>MGPIPPTGVPVGDFFVCGRMTTLHMGGQSGIQATTLVNGMIYRTDHPEPSTSPVSNWEFTVLENNTIVGAGMGCVWFQKSEALVWTLDGQKLSGWNTLDGVGTTQLTVAWRQHNRTIYGWANVVAWNSEEWHTNAEQPHQPILRLTYWLVKINVLSEPEDFDVVQKSPLAYLEDYTTAQSKSAIQKLNFQTFQKPEGGGTLRAQYSTTPRQGDFAVIWQIGRHNFDMSTGKGTPVESLSDYVMPQQ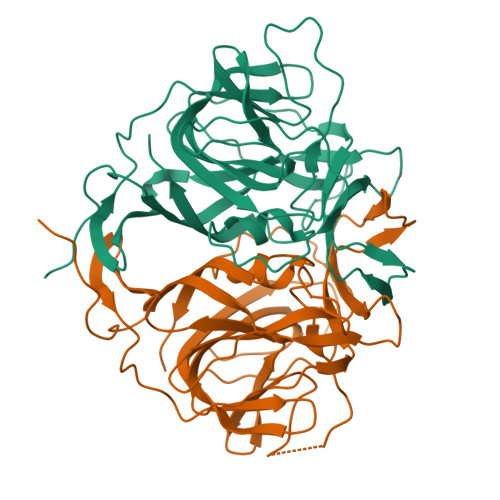KDAHIGMWYRALTSVGPRTDVLTLHFHLPTVEKAAAELALVPR[2x]> MASWSHPQFEKGGTHVAETSAPTRSEPDTRVLTLPGTASAPEFRLIDIDGLLNNRATTDVRDLGSGRLNAWGNSFPAAELPAPGSLITVAGIPFTWANAHARGDNIRCEGQVVDIPPGQYDWIYLLAASERRSEDTIWAHYDDGHADPLRVGISDFLDGTPAFGELSAFRTSRMHYPHHVQEGLPTT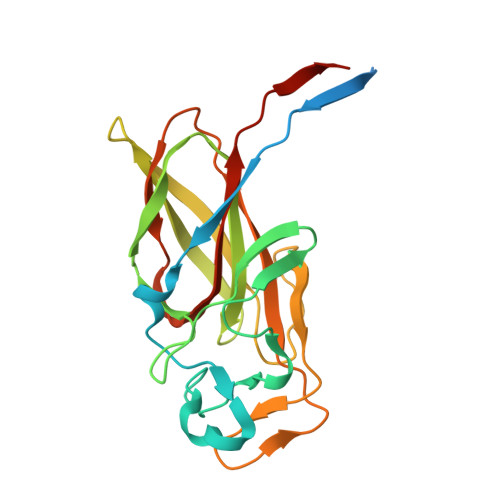MWLTRVGMPRHGVARSLRLPRSVAMHVFALTLRTAAAVRLAEGATT>MSKKEININNYNDDAIQVLEGLDAVRKRPGMYIGSTDGAGLHHLVWEIVDNAVDEALSGFGDRIDVTINKDGSLTVQDHGRGMPTGMHAMGIPTVEVIFTILHAGGKFGQGGYKTSGGLHGVGSSVVNALSSWLEVEITRDGAVYKQRFENGGKPVTTLKKIGTAPKSKTGTKVTFMPDATIFSTTDFKYNTISERLNESAFLLKNVTLSLTDKRTDEAIEFHYENGVQDFVSYLNEDKEILTPVLYFEGEDNGFQVEVALQYNDGFSDNILSFVNNVRTKDGGTHETGLKSAITKVMNDYARKTGLLKEKDKNLEGSDYREGLAAVLSILVPEEHLQFEGQTKDKLGSPLARPVVDGIVADKLTFFLMENGELASNLIRKAIKARDAREAARKARDESRNGKKNKKDKGLLSGKLTPAQSKNPAKNELYLVEGDSAGGSAKQGRDRKFQAILPLRGKVINTAKAKMADILKNEEINTMIYTIGAGVGADFSIEDANYDKIIIMTDADTDGAHIQTLLLTFFYRYMRPLVEAGHVYIALPPLYKMSKGKGKKEEVAYAWTDGELEELRKQFGKGATLQRYKGLGEMNADQLWETTMNPETRTLIRVTIEDLARAERRVNVLMGDKVEPRRKWIEDNVKFTLEEATVFHMSNIQNMSLEDIMGERFGRYSKYIIQDRALPDIRDGLKPVQRRILYSMNKDSNTFDKSYRKSAKSVGNIMGNFHPHGDSSIYDAMVRMSQNWKNREILVEMHGNNGSMDGDPPAAMRYTEARLSEIAGYLLQDIEKKTVPFAWNFDDTEKEPTVLPAAFPNLLVNGSTGISAGYATDIPPHNLAEVIDAAVYMIDHPTAKIDKLMEFLPGPDFPTGAIIQGRDEIKKAYETGKGRVVVRSKTEIEKLKGGKEQIVITEIPYEINKANLVKKIDDVRVNNKVAGIAEVRDESDRDGLRIAIELKKDANTELVLNYLFKYTDLQINYNFNMVAIDNFTPRQVGIVPILSSYIAHRREVILARSRFDKEKAEKRLHIVEGLIRVISILDEVIALIRASENKADAKENLKVSYDFTEEQAEAIVTLQLYRLTNTDVVVLQEEEAELREKIAMLAAIIGDERTMYNLMKKELREVKKKFATPRLSSLEDTAKALEHHHHHH[2x]

Topoisomerase (topo) IV and gyrase are the type II enzymes expressed in bacteria. Topo IV mediates the unlinking of daughter chromosomes before cell division, whereas gyrase is unique in its ability to introduce negative supercoils into DNA thereby controlling chromosome supercoiling, which promotes replication fork advance and allows global regulation of gene expression. In each case, the active complex is a tetramer of two topo IV ParC and ParE subunits or gyrase GyrA and GyrB proteins. By contrast, the N-terminal and C-terminal regions of the highly conserved ParE (GyrB) subunits form the ATPase- and Mg2+-binding-TOPRIM domains, respectively.

First, to prevent subunit dissociation and generate a stabilized complex, we engineered a catalytically active fusion protein comprising the full-length ParE and breakage-reunion ParC55 domain. Second, we used an alternative gate-DNA, namely, a 34mer DNA duplex comprising the plasmid V-site, which we have shown is also strongly cleaved by pneumococcal topo IV (Arnoldi ref). Co-crystallization of the fusion protein with a 2.2-fold excess of V-site DNA yielded a crystal structure in space group P42212 with the best resolution of 3.7 Å. This new structure reveals a novel (ParE-ParC55)2 dimer complex bound to two DNA molecules and adopting the open clamp conformation (open ParE N-gate; closed G and C gates). The DNA bound at the G-gate is bent and uncleaved and adopts an A-form conformation immediately at the scission sequence while retaining B-form on the flanks for drug-free DNA complexes of ParC55 with ParE30 (19). By contrast, the second DNA molecule links each of four complexes together within the crystal lattice by binding to the long helices of the C-gate via ParC R468, K464, N461 and H196 residues and is entirely in the linear unbent B-form. The presence of a second DNA-binding site on ParC has not been reported previously, and its unveiling is most likely a consequence of the higher ratio of DNA used in the crystallization conditions. The complex was crystallized in the absence of ATP and reveals novel aspects of the open N-gate conformation. The two N-terminal ParE ATPase domains (residues 1–399 shown in red in Figure 3) (that dimerize on ATP binding to close the N-gate) are located far apart fully exposing the G-segment (in green) to the solvent from above. In our structure, the ATP binding site is empty and covered by the neighbouring α-helix from the same ParE monomer, plausibly protecting it from ATP binding before T-segment capture, a feature not previously observed in other crystal structures of the ATPase domains of ParE and GyrB dimers. The link is mobile and poorly ordered, so its exact fold is not evident from the crystallographic data.>[2x]PLREAKDLHTALHIGPRALSKASNISMQQAREVVQTCPHCNSAPALEAGVNPRGLGPLQIWQTDFTLEPRMAPRSWLAVTVDTASSAIVVTQHGRVTSVAVQHHWATAIAVLGRPKAIKTDNGSCFTSKSTREWLARWGIAHTTGIPGNSQGQAMVERANRLLKDKIRVLAEGDGFMKRIPTSKQGELLAKAMYALNHKERGENTKTPIQKHWRPTVLTEGPPVKIRIETGEWEKGWNVLVWGRGYAAVKNRDTDKVIWVPSRKVKPDIT

The following permanent integration of this viral DNA by the viral-encoded integrase (IN) into the host chromosome is a necessary step in virus replication. In most retrovirus systems, IN first removes a dinucleotide from both termini of the linear blunt-ended viral DNA (∼10 kb), termed 3′ OH processing. Next, the same active sites catalyze the concerted transesterification reactions of the nascent 3′ OH groups into the cell DNA. RSV IN consists of the N-terminal domain (NTD) (residues 1–44), the catalytic core domain (CCD) (residues 50–214), and the C-terminal domain (CTD) (residues 222–286), similar in size to the corresponding domains of HIV IN.

Although many crystal structures are available for single or two-domain fragments of HIV, RSV, simian immunodeficiency virus, and bovine immunodeficiency virus IN [22], a three-domain retroviral IN complete with all structural domains has not been characterized using x-ray crystallography. Earlier crystallographic and NMR studies showed that the extreme C-terminal region of RSV IN spanning residues 271–286, and the corresponding residues 271–288 of HIV IN, are disordered. Thus, we generated RSV IN(1–270) lacking this flexible C-terminal “tail”. We have obtained crystals of the three-domain RSV IN(1–270) in several different conditions. Although the crystals typically grew as very thin needles not useful for x-ray diffraction experiments, the crystal morphology was improved by seeding and introducing protein mutations. Diffraction quality crystals were obtained in the presence of a solubility-enhancing F199K mutation. We demonstrated here that RSV IN 1–270 possesses the same capacity in vitro for 3′ OH processing and concerted integration as the wild type RSV IN (1–286). A possible explanation would be that the residue F199 interacts with the NTD of RSV IN to mediate IN tetramerization during the concerted integration reaction. As RSV IN residue L8 aligns with E11 of HIV IN, a hydrophobic interaction between L8 and F199 might play a role in RSV IN tetramerization. Taken together, these results imply that the CCD and CTD of RSV IN are primarily responsible for viral and target DNA binding whereas the NTD is essential for IN tetramerization required for concerted integration.> MKKLVFTFKRIDHPAQDLAVKFHGFLMEQLDSDYVDYLHQQQTNPYATKVIQGKENTQWVVHLLTDDHEDKVFMTLLQIKEVSLNDLPKLSVEKVEIQELGADKLLEIFNSEENQTYFSIIFETPTGFKSQGSYVIFPSMRLIFQSLMQKYGRLVENQPEIEEDTLDYLSEHSTITNYRLETSYFRVHRQRIPAFRGKLTFKVQGAKTLKAYVKMLL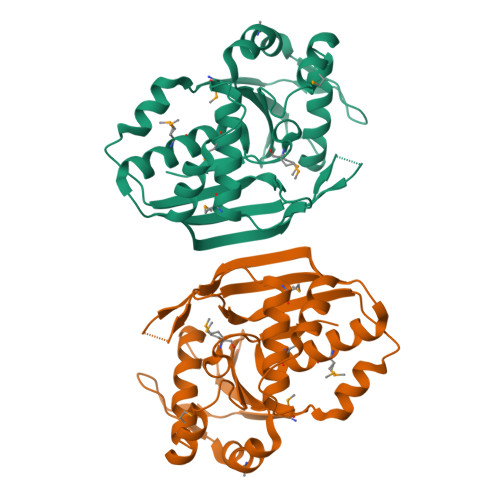TFGEYSGLGMKTSLGMGGIKLEERKD> MALKGN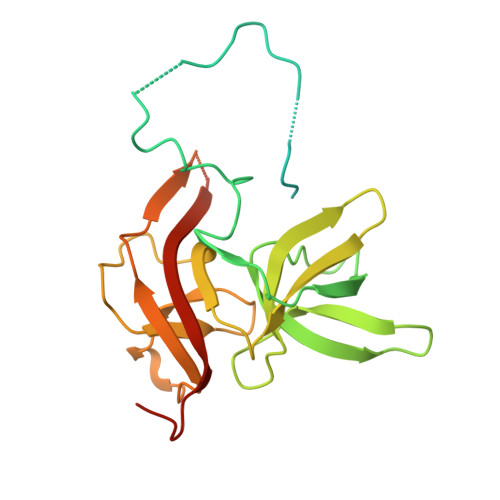MQVENLEAVEDPQVDLGAQVSAAPRAKRQARQAEDVQGEDPYLESISELDDVLLKFKKYSKSMSSIENKVFSSSSGCFKSKNERVDAYSFACSSYTDKIEEYLYDPANSFPYKRGVKLVPKENSIYVEVGADTDMYGICVDVCEFSCTAYVLPITNNFEGYLVTRNPSIKIGEILDINNNGVIIKAGGGPPTAINIYALSDSFTINFAPEDGNQDQNRYPRQEYSINLIKVAIFGNRGLEKTVNPDGG BV IXα is then the substrate for many members of the ferredoxin-dependent bilin reductases (FDBRs) that catalyze a regio- and stereospecific reduction of the tetrapyrrole pigment. However, during the reaction, a second aspartate residue gets involved and likely serves as a proton donor for the proton coupled electron transfer to the A-ring of the tetrapyrrole molecule. This reaction catalyzed by PebB is a formal reduction of the 2,3,31,32-dien system of the A-ring of 15,16-DHBV. Here we solved the crystal structure of the PebB homolog PEBB (nuclear encoded proteins in eukaryotes are denoted with capital letters by convention) from the eukaryotic cryptophyte alga Guillardia theta. The eukaryotic mGtPEBB is a globular single domain protein that shows the characteristic FDBR α/β/α-sandwich fold with a central antiparallel β-sheet, flanked by α-helices.

The substrate-free model of mGtPEBB was used to determine the structure of the mGtPEBB–DHBV complex, which crystallized in space group P21 with two molecules in the asymmetric unit. Both chains showed clear density for DHBV already after molecular replacement, even though chain A had overall higher B-values and somewhat lower occupancy of the substrate. Electron density for the vinyl groups defined the orientation of the substrate in both chains. DHBV is bound in a niche formed by the central β-sheet on the proximal and by helices H6/H7 on the distal side of the substrate. Although Asp-219 coordinates a central pyrrole water molecule, Asp-99 is in direct contact with the substrate and coordinates the polar pyrrole nitrogen of the D-ring and the carbonyl oxygen of the A-ring. In our crystal structure, Asp-99 had to be modeled in alternate conformations. Because the mGtPEBB–DHBV crystals were grown at pH 8.5 and appeared in similar purple color, the observed alternate conformations most likely reflect this deprotonation of Asp-99. Contrary to this hypothesis, we identified a flipped binding orientation of DHBV in GtPEBB based on strong density for the vinyl groups. This results in an inverted positioning of the A- and D-rings. In addition, although the ligand adopts a planar conformation with three of its pyrrole rings, one pyrrole ring is tilted out of the plane.

>GGSEAVSDIYKPFWEWAAKTIKERLGDDLVSYPIPDGYLRKEAMVGKGKRESLAWTQSYGYQTKKMRQIRAAHVNGGASLQVLNLVFFPHMNYDLPFLGLDLVTLPGGHLIAIDMQPLFQTEEYKKKYAEPCMDMYQKHVKNLPWGGDFPEEAKQYFSPVFLWTRPQEDKQVETYVFEAFKDYINKYLDFVEAAKPVTDPDHLARIRERQLSYLQYRAEKDPARGMFTRMYGPEWTERYIHGFLFDLEEKMESGEYKTGELLPCSDPLNFQPTPL[2x]The CTLH (C-terminal to lissencephaly-1 homology motif) complex is a multisubunit RING E3 ligase with poorly defined substrate specificity and flexible subunit composition. Besides the reciprocal incorporation of Wdr26 and muskelin, another known alternative assembly path of the CTLH complex involves the mutually exclusive incorporation of the Armc8α subunit or its shorter isoform Armc8β (673 versus 399 residues). Both subunits share the first 378 residues comprised of seven Armadillo repeat motifs. The remaining scaffolding subunits, Armc8β and Twa1, strongly interact with each other and with RanBP9, again with nanomolar affinity.

To identify possible oligomerization sites, we solved the crystal structure of Armc8β after crystallization of selenomethionine-labeled protein by single-wavelength anomalous diffraction at the selenium edge and refined the structure at a resolution of 2.7 Å. The crystals contained three chains (denoted as p, i, and a) in the asymmetric unit. Remarkably, each copy exhibited a distinct conformation, thus demonstrating dynamic flexibility of Armc8β especially at its termini. Chains p and a are more similar as reflected in an rms deviation of 1.04 Å after superimposition of the Cα atoms of all modeled residues, whereas chain i adopts a more compact shape; in this case, the rms deviations are 2.82 Å for the ia pair and 1.69 Å for the ip pair. In terms of oligomerization sites, analysis of the structure with the PISA server detected no significant stable assembly, which is in line with the dynamic nature of Armc8β′s oligomerization behavior. Apparently, the high concentrations in the crystal promoted the observed interactions, nevertheless, since chain p shares an interface with both chain i and chain a, it is tempting to speculate that these two interaction sites could correspond to the two sites identified when analyzing the self-association of Armc8β by SEC–MALS. Not surprisingly, the overall fold of Armc8α and its shorter isoform Armc8β are very similar. However, in our structure we could model an additional short α-helix at the N terminus. The conformation which Armc8α adopts in the complex is more closely related to the less bent conformation observed for chains a (rms deviation of 0.93 Å) or p (rms deviation of 1.05 Å) of Armc8β, than to chain i (rms deviation of 1.94 Å). Human and mouse Armc8α are very closely related (overall identity of 98.51% with only two substitutions in the crystallized region), and the C-termianl extension, which is unique to Armc8β, is very flexible and therefore could only be partially resolved (5–9 residues). It is more likely that structural differences arise because Armc8α is being present in a complex, whereas Armc8β was analyzed in isolation.

>[3x]MACLLETPIRMSVLSEVTASSRHYVDRLFDPDPQKVLQGVIDMKNAVIGNNKQKANLIVLGAVPRLLYLLQQETSSTELKTECAVVLGSLAMGTENNVKSLLDCHIIPALLQGLLSPDLKFIEACLRCLRTIFTSPVTPEELLYTDATVIPHLMALLSRSRYTQEYICQIFSHCCKGPDHQTILFNHGAVQNIAHLLTSPSYKVRMQALKCFSVLAFENPQVSMTLVNVLVDGELLPQIFVKMLQRDKPIEMQLTSAKCLTYMCRAGAIRTDDSCIVLKTLPCLVRMCSKERLLEERVEGAETLAYLIEPDVELQRIASITDHLIAMLADYFKYPSSVSAITDIKRLDHDLKHAHELRQAAFKLYASLGANDEDIRKKIIVSLGEGRPPVLTASRQGVTST> SVTSAKVAVNGVQLHYQQTGEGDHAVLLLPGMLGSGETDFGPQLKNLNKKLFTVVAWDPRGYGHSRPPDRDFPADFFERDAKDAVDLMKALKFK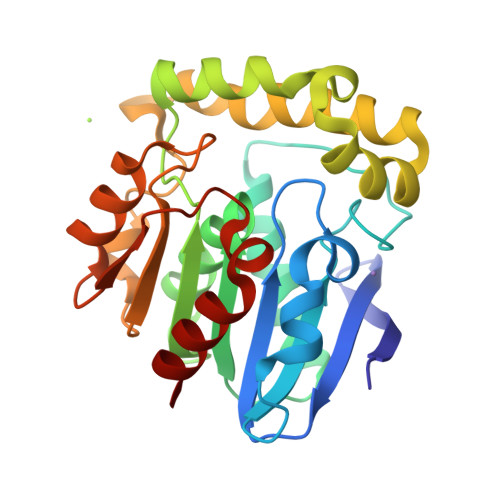KVSLLGWSNGGITALIAAAKYPSYIHKMVIWGANAYVTDEDSMIYEGIRDVSKWSERTRKPLEALYGYDYFARTCEKWVDGIRQFKHLPDGNICRHLLPRVQCPALIVHGEKDPLVPRFHADFIHKHVKGSRLHLMPEGKHNLHLRFADEFNKLAEDFLQ>VTRNVEVTAEEEKIRDKLGYEAIRDIHRDMDDDHSGSIDRNESTGFMKEDMQMRGSERTRRENKFHGDDDAITVDDLWEAWFESIERTWTNERLVEWLINDVNLPSIVEAVKAKKIDGKILPRFASPNSDFLNK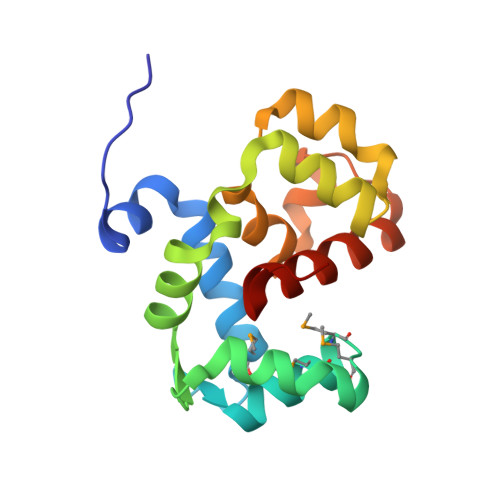ELGIKSSVYRQKLRLNSLDVVLFGYKD[2x]> GSSHHHHHHSQDLMASQHSPTPVKVPAAAANYTPATLDQDLRSQINSLLIKEGHVAKIQEHLLHHLHAHPSNWPTVVQNHALSLLRSGEVTSFPALLRRVVEDVRQDTALAPSSTTANGNGESTTTNGATNGKGA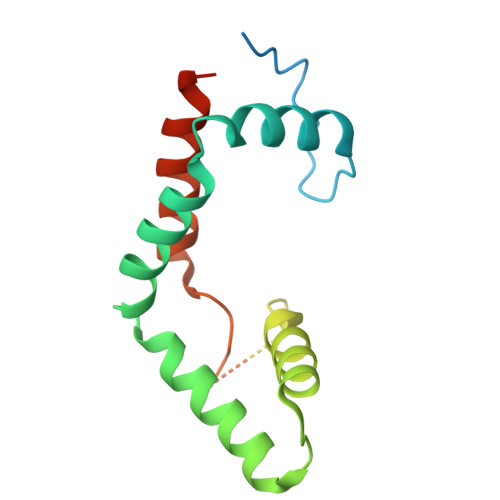TTNGNKGGVADLKPSLAVPQSVVEEALKVTRECLDQLCEIEEPLAA> MSSRKSTASSLLLRQYRELTDPKKAIPSFHIELEDDSNIFTWNIGVMVLNEDSIYHGGFFKAQMRFPEDFPFSPPQFRFTPAIYHPNVYRDGRLCISILHQSGDPMTDEPDAETWSPVQTVESVLISIVSLLEDPNINSPANVDAAVDYRKNPEQYKQRVKMEVERSKQDIPKGFIMPTSE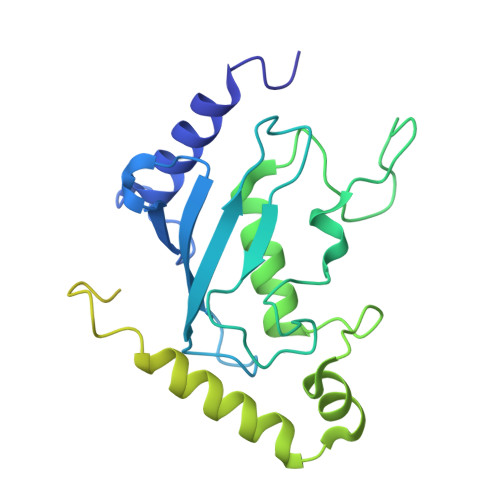SAYISQSKLDEPESNKDMADNFWYDSDLDDDENGSVILQDDDYDDGNNHIPFEDDDVYNYNDNDDDDERIEFEDDDDDDDDSIDNDSVMDRKQPHKAEDESEDVEDVERVSKKI4-{[(3S)-1-{7-[(3,4-dimethoxyphenyl)amino][1,3]thiazolo[5,4-d]pyrimidin-5-yl}pyrrolidin-3-yl]carbamoyl}benzoic acid | C25 H24 N6 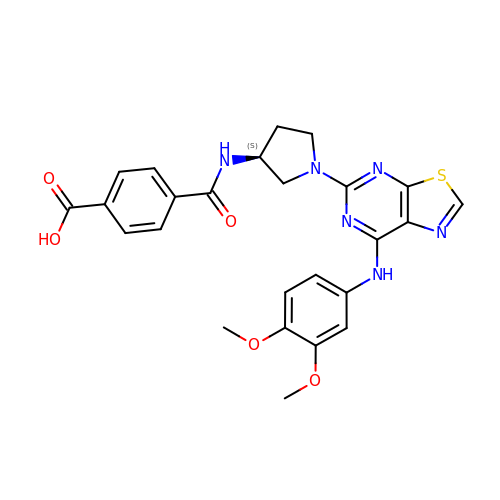O5 S | GRGCZORIQMQMAN-KRWDZBQOSA-N> AQLTIEAVPSNAAEGKEVLLLVHNLPQDPRGYNWYKGETVDANRRII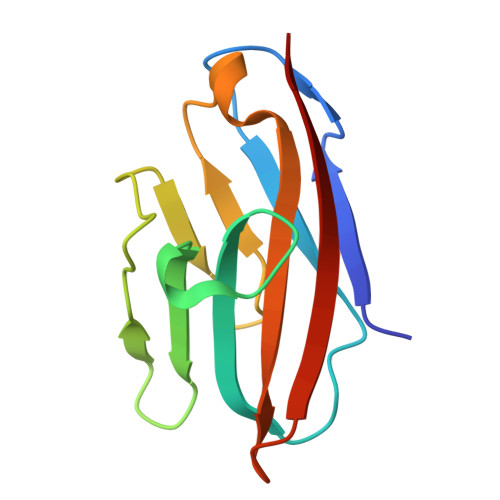GYVISNQQITPGPAYSNRETIYPNASLLMRNVTRNDTGSYTLQVIKLNLMSEEVTGQFSVH> LMGCVAETPPRFTRTPVDQTGVSGGVASFICQATGDPRPKIVWNKKGKKVSNQRFEVIEFDDGSGSVLRIQPLRTPRDEAIYECVASNNVGEISVSTRLTVLREDQIPRGFPTIDMGPQLKVVERTRTATMLCAASGNPDPEITWFKDFLPVDTSNNNGRIKQLRSESIGGTPIRGALQIEQSEESDQGKYECVATNSAGTRYSAPANLYVRELREVRRVPPRFSIPPTNHEIMPGGSVNITCVAVGSPMPYVKWMLGAEDLTPEDDM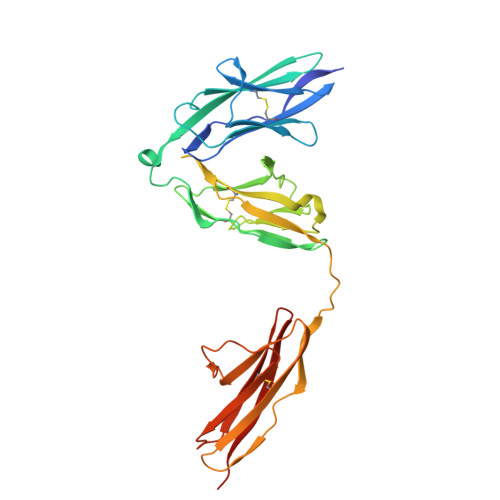PIGRNVLELNDVRQSANYTCVAMSTLGVIEAIAQITVKAHHHHHH>[4x]MKYMI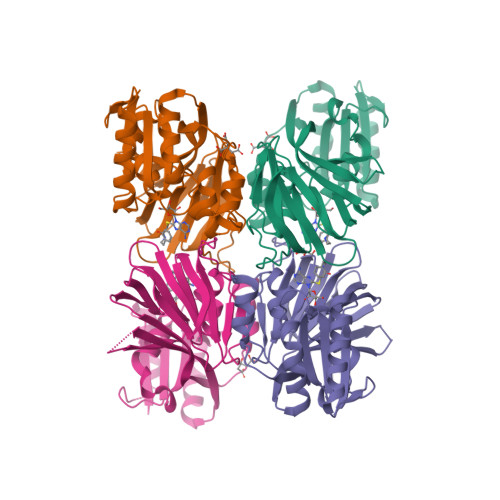TSKGDEKSDLLRLNMIAGFGEYDMEYDDVEPEIVISIGGDGTFLSAFHQYEERLDEIAFIGIHTGHLGFYADWRPAEADKLVKLLAKGEYQKVSYPLLKTTVKYGIGKKEATYLALNESTVKSSGGPFVVDVVINDIHFERFRGDGLCMSTPSGTTAYNKSLGGALMHPSIEAMQLTEMASINNRVYRTIGSPLVFPKHHVVSLQPVNDKDFQISVDHLSILHRDVQEIRYEVSAKKIHFARFRSFPFWRRVHDSFIEDLEHHHHHH(9Z)-11-{hydroxy[(5S)-6-{[(1S)-3-{[(3S)-1-hydroxy-2-oxoazepan-3-yl]amino}-1-methyl-3-oxopropyl]oxy}-5-({[(4S)-2-(2-hydroxyphenyl)-4,5-dihydro-1,3-oxazol-4-yl]carbonyl}amino)-6-oxohexyl]amino}-11-oxoundec-9-enoic 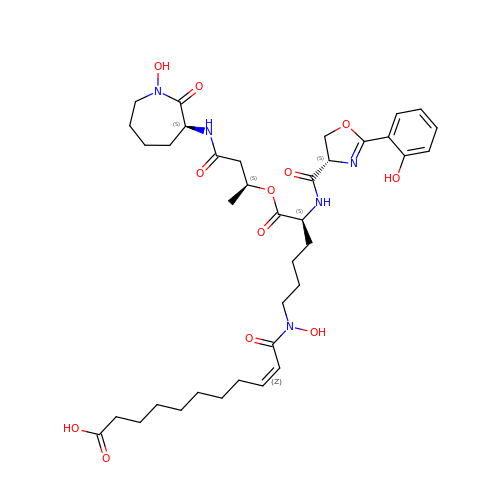acid | C37 H53 N5 O12 | DRNVRDPDTBNRNR-SFCJKLQFSA-N Inteins catalyze their removal from a host protein through protein splicing. The HINT domain catalyzes the protein splicing reaction, whereas HEN domains often function independently of the HINT domain. In this study, we elucidated crystal structures of HEN-associated archaeal inteins inserted at the same insertion site (VMA-b), which is located within the A subunit P-loop of the vascular-type ATP synthase (VMA) from Thermococcus litoralis (Tli) and Pyrococcus horikoshii (Pho). The two three-dimensional structures highlighted a modular architecture consisting of HINT, HEN, and an accessory domain (ACD).

Among VMA inteins inserted at the VMA-b insertion site, we could obtain crystals of the VMA intein from Thermococcus litoralis (Tli). The TliVMA intein comprises 429 residues and is larger than the PhoVMA intein (376 residues) but similar to the size of PI-SceI (454 residues). To prevent self-cleavages during protein production, we expressed both inteins in E. coli with alanine substitutions of the catalytic cysteines 1 (Cys1). We solved the structure of TliVMA intein at the 1.6 Å-resolution. The crystal structures of the TliVMA intein revealed a very similar overall structure as found in the PhoVMA intein, including the three-domain architecture known from the three other reported HEN-containing inteins. The HINT domain of the TliVMA intein also contains the β-strand extension found among thermophilic inteins. However, TliVMA intein probably carries a catalytically active HEN domain capable of binding to DNA and introducing DNA double-strand breaks. Indeed, we observed that TliVMA intein cleaved its reconstituted homing site accompanied by a strong DNA binding affinity as indicated by an electrophoretic mobility shift (EMSA) of the substrate- and product-DNA fragments. Our results demonstrated that the ACD in TliVMA intein induced a second cleavage site in addition to the theoretical homing site. The ACD of TliVMA intein strongly resembles the helix-turn-helix motif common for many DNA binding proteins, such as transcriptional regulator proteins.

> SGKAVDGNTLVLTEEFGLVKIKELYEKLDGKGRKTVEGNEEWTELETPVTVYGYRNGRIVGIKATHIYKGISSGMIEIRTRTGRKIKVTPIHKLFTGRVTKDGLALEEVMAMHIKPGDRIAVVKKIDGGEYVKLTTSPDFRKSRKIKVPEVLDEDLAEFLGYLIADGTLKPRTVAIYNNDESLLKRANFLSTKLFGINGKIVQERTVKALLIHSKPLVDFFRKLGIPESKKARNWKVPRELLLSPPSVVKAFINAYIVCDGYYHERKGEIEITTASEEGAYGLSYLLAKLGIYATFRKKQIKGKEYYRIAISGKTNLEKLGIKRETRGYTNIDIVPVEVESIYNALGRPYSELKGEGIEIHNYLNGENMTYETFRKFAKLVGLEEVAENHLKHILFDEVVEVKYIPEPQEVYDITTETHNFVGGNMPTLLHN N-[(1S,2R)-1-benzyl-2-hydroxy-3-{[3-(trifluoromethyl)benzyl]amino}propyl]-7-ethyl-1-methyl-3,4-dihydro-1H-[1,2,5]thiadiazepino[3,4,5-hi]indole-9-carboxamide 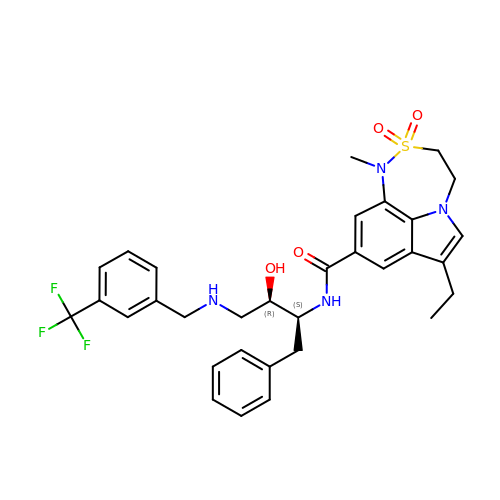2,2-dioxide | C32 H35 F3 N4 O4 S | MSHYGGHZTGSTOG-LMSSTIIKSA-N> MLDINAFLVEKGGDPEIIKASQKKRGDSVELVDEIIAEYKEWVKLRFDLDEHNKKLNSVQKEIGKRFKAKEDAKDLIAEKEKLSNEKKEIIEKEAEADKNLRSKINQVGNIVHESVVDSQDEENNELVRTWTPENYKKPEQIAAATGAPAKLSHHEVLLRLDGYDPERGVRIVGHRGYFLRNYGVFLNQALINYGLLFLSSKGYVPLQAPVMMNKEVMAKTAQLSQFDEELYKVIDGEDEKYLIATSEQPISAYHAGEWFESPAEQLPVRYAGYSSCFRREAGSHGKDAWGIFRVHAFEKIE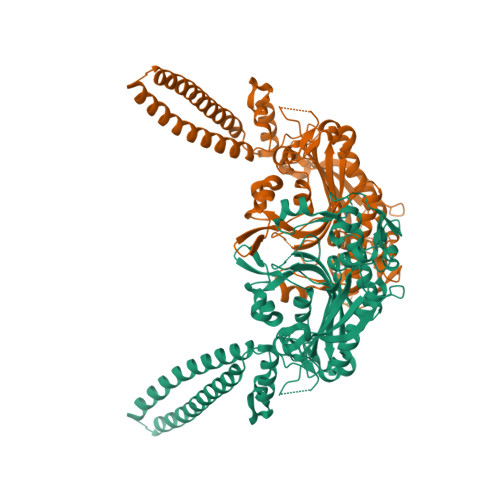QFVLTEPEKSWEEFDRMIGCSEEFYQSLGLPYRVVGIVSGELNNAAAKKYDLEAWFPFQQEYKELVSCSNCTDYQSRNLEIRCGIKQQNQQEKKYVHCLNSTLSATERTICCILENYQKEDGLVIPEVLRKYIPGEPEFIPYIKELPKNTTSVKKAKGKNPKNTTSVKKAKGKNGSRHHHHHH>[2x]TNLLPNIKEDKMLTLRREIKSPSKSALDSFTLIMQTYNRTDLLLRLLNHYQAVPSLHKVIVVWNNVGEKGPEELWNSLGPHPIPVIFKPQTANKMRNRLQVFPEVETNAVLMVDDDTLISAQDLVFAFSIWQQFPDQIIGFVPRKHVSTSSGIYSYGGFELQTPGPGNGDQYSMVLIGASFFNSKYLEL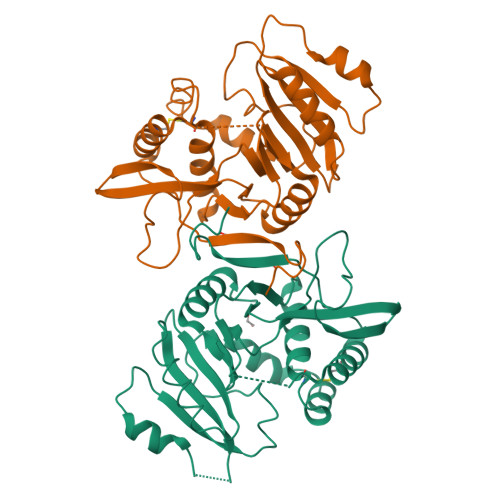FQKQPAAVHALIDETQNCDDIAMNFLVTRHTGKPSGIFVKPINMVNLEKETNGYSGMWHRAEHFLQRSYCINKLVNIYDGMPLKYSNIMISQFGFPYANHKSKM>[2x]QTVTEPVGSYARAERPQDFEGFVWRLDNDGKEALPRNFRTSADALRAPEKKFHLDAAYVPSREGMDALHISGSSAFTPAQLKNVAAKLREKTAGPIYDVDLRQESHGYLDGIPVSWYGERDWANLGKSQHEALADERHRLHAALHKTVYIAPLGKHKLPEGGEVRRVQKVQTEQEVAEAAGMRYFRIAATDHVWPTPENIDRFLAFYR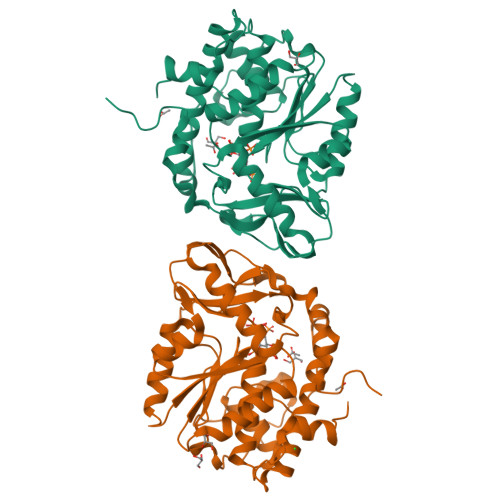TLPQDAWLHFHSEAGVGRTTAFMVMTDMLKNPSVSLKDILYRQHEIGGFYYGEFPIKTKDKDSWKTKYYREKIVMIEQFYRYVQENRADGYQTPWSVWLKSHPAKA> SSFEGQMAEYPTISIDRFDRENLRARAYFLSHCHKDHMKGLRAPTLKRRLECSLKVYLYCSPVTKELLLTSPKYRFWKKRIISIEIETPTQISLVDEASGEKEEIVVTLLPAGHCPGSVMFLFQGNNGTVLYTGDFRLAQGEAARMELLHSGGRVKDIQSVYLDTTFCDPRFYQIPSREECLSGVLELVRSWITRSPYHVVWLNCKAAYGYEYLFTNLSEELGVQVHVNKLDMFRNMPEILHHLTTDRNTQIHACRHPKAEEYFQWSKLPCGITSRNRIPLHIISIKPSTMWFGERSRKTNVIVRTGESSYRACFSFHSSYSEIKDFLSYLCPVNAYPNVIPVGTTMDKVVEILKPLCRSSQSTEPKKGENLYFQ

Artemis (SNM1C/DCLRE1C) is an endonuclease that plays a key role in development of B- and T-lymphocytes and in dsDNA break repair by non-homologous end-joining (NHEJ). Artemis is phosphorylated by DNA-PKcs and acts to open DNA hairpin intermediates generated during V(D)J and class-switch recombination. Artemis belongs to a superfamily of nucleases containing metallo-β-lactamase (MBL) and β-CASP (CPSF-Artemis-SNM1-Pso2) domains. The overall fold of the catalytic core of Artemis is similar to that of SNM1A and SNM1B (2 Å backbone RMSD); it has all the key structural characteristics of human MBL fold nucleases, with the di-metal containing active site at the interface between the MBL and β-CASP domains.

A striking aspect of the reported structures is that both crystal forms were obtained in the presence of DNA and were reported to require DNA for their growth; the crystals showed a fluorescence signal supporting the presence of DNA (the oligonucleotides used contained a cyanine dye fluorophore), yet neither of the models presented contain DNA. We re-examined these structures looking closely at the residual electron density. The model contains an 8-nucleotide 5′-single-stranded extension with a short 2-base pair region of duplex DNA that reaches into the Artemis active site, making close contacts with the metal ion centre in a manner consistent with the proposed catalytic mechanism. The sequence of the longest strand corresponds to the 10-nucleotide cy-5 labelled strand (cy5-GCGATCAGCT) with residual density at the 5′-end that may be attributed to the cyanine fluorophore which we did not include in our model. The complementary strand used in crystallization was 13-nucleotides long and was intended to produce a 5′-overhang, but only two bases and three phosphates could be located in the density. The abrupt manner in which the electron density apparently disappears from either end of this strand suggests that this is the product of a cleavage reaction, although it is possible that remaining nucleotides are not located due to disorder. The analysis of electron density at this site is complicated by the proximity to a crystallographic 2-fold symmetry axis, which brings a symmetry copy of the DNA molecule into a position where atoms partially overlap and the extended 5′ strands form a pseudo duplex. The occupancy of the entire DNA molecule is thus limited to 0.5, and the lower occupancy is reflected in the electron density map which requires a lower contour level than would usually be applied. After carefully building and refining the afore-described DNA bound model, significant positive electron density was revealed for the second metal ion (M2 site) which we included in the model with the same occupancy (0.5) as the DNA. Thus, our model suggests Artemis preferentially binds DNA with a 5′-overhang binding at the junction between double- and single-stranded regions; the expected product of this reaction would be a blunt ended DNA with a 5′-phosphate.> EDDWSKPLPPSERLEQELFSGGNTGINFEKYDDIPVEATGNNCPPHIESFSDVEMGEIIMGNIELTRYTRPTPVQKHAIPIIKEKRDLMACAQTGSGKTAAFLLPILSQIYSDGPGEALRAMKENGRYGRRKQYPISLVLAPTRELAVQIYEEARKFSYRSRVRPCVVYGGADIGQQIRDLERGCHLLVATPGRLVDMMERGKIGLDFCKYLVLDEADRMLDMGFEPQIRRIVEQDTMPPKGVRHTMMFSATFPKEIQMLARDFLDEYIFLAVGRVGSTSENITQKVVWVEESDKRSFLLDLLNATGKD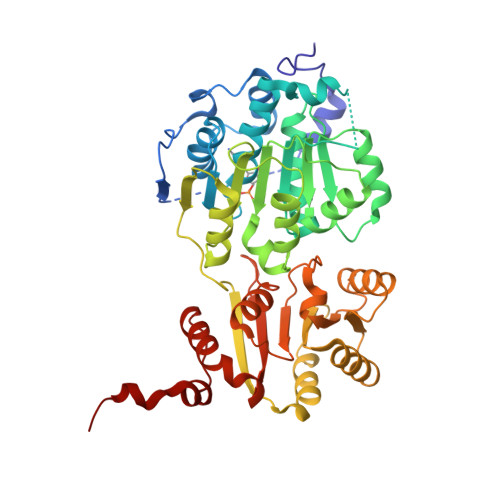SLTLVFVETKKGADSLEDFLYHEGYACTSIHGDRSQRDREEALHQFRSGKSPILVATAVAARGLDISNVKHVINFDLPSDIEEYVHRIGRTGRVGNLGLATSFFNERNINITKDLLDLLVEAKQEVPSWLENMAYEHHYKGSS>SDLDHDLSVKKQELIESISRKLQVLREARESLLEDVQANTVLGAEVEAIVKGVCKPSEFDKFRMFIGDLDKVVNLLLSLSGRLARVENALNNLDDGASPGDRQSLLEKQRVLIQQHEDAKELKENLDRRERIVFDILAN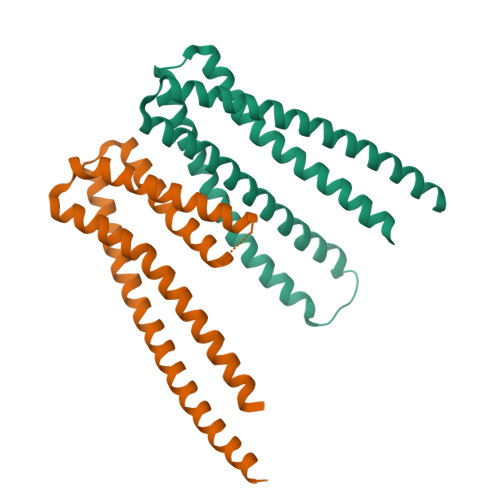YLSEESLADYEHFVKMKSALIIEQRELEDKIHLGEEQLKCLLDSL[2x]tert-butyl 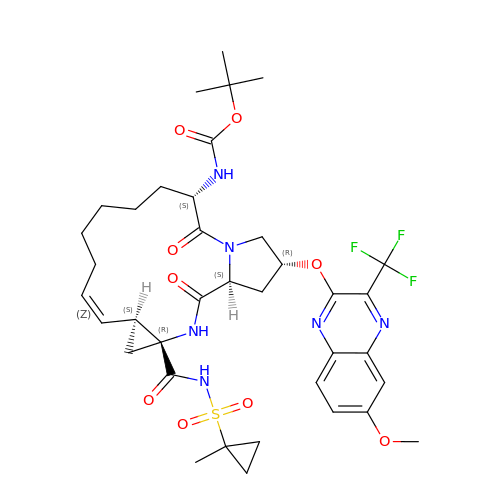[(2R,6S,12Z,13aS,14aR,16aS)-2-{[6-methoxy-3-(trifluoromethyl)quinoxalin-2-yl]oxy}-14a-{[(1-methylcyclopropyl)sulfonyl]carbamoyl}-5,16-dioxo-1,2,3,5,6,7,8,9,10,11,13a,14,14a,15,16,16a-hexadecahydrocyclopropa[e]pyrrolo[1,2-a][1,4]diazacyclopentadecin-6-yl]carbamate | C37 H47 F3 N6 O9 S | IYYDCFFQTJJOBE-NTPKMKHWSA-N N-(4-chlorobenzyl)-5-(furan-2-yl)-1H-1,2,4-triazol-3-amine | C13 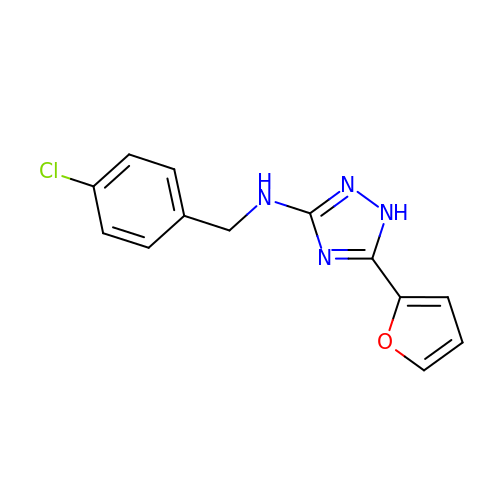H11 Cl N4 O | IRHUOSKJHRHZKH-UHFFFAOYSA-N Vibrio cholerae contains multiple copies of chemotaxis response regulator (VcCheY1–VcCheY4) whose functions are elusive yet. Autophosphorylated CheA then donates phosphate to the response regulator CheY. Phosphorylated CheY interacts with the flagellar motor protein FliM and influence the direction of flagellar rotation from counter clock wise (CCW) to clock wise (CW). As expected, both VcCheY3 and VcCheY4 possess (β/α)5 fold typical of the response regulators.

VcCheY4 was crystallized in two different states; one is in free state with no ligand attached (VcCheY4free) and another with a sulfate and a Ca2+ ion bound at the active site (VcCheY4sulf). In contrast to that, neither a metal ion nor a sulfate ion was observed at the active site of VcCheY4free although both of these components were added during crystallization. Absence of the divalent metal ion do not cause any change in the side chain conformation of D9 and D52 compared to VcCheY4sulf, but the carbonyl oxygen of N54 points away from the metal binding side. As a result, the β3α3 loop of VcCheY4free takes a different conformation and moves about 3 Å away from the active site. In VcCheY4free, helix α4 is shorter and β4α4 loop is unusually longer compared to those of VcCheY4sulf. The plot of B′-values indicated that the crystallographic B-factor of the β4α4 loop is much lower in VcCheY4sulf compared to that of VcCheY4free. Interestingly, when VcCheY4free is superposed on VcCheY4sulf significant differences are observed at the active site, together with helix α4, β4α4 loop and β3α3 loop. Our packing analysis suggests that, in either case, these regions are rather loosely packed and their conformations are not influenced by crystal packing. The crucial residue at β5 that acquires ‘in’ position upon activation is a Trp (W101) in case of VcCheY4 and in both the structures of VcCheY4 the side chain of W101 acquired ‘in’ position. In fact, this is the first structure of a naturally occurring CheY where Trp at this crucial position is observed to spontaneously occupy ‘in’ position, even without activation.

> TMAKVLAVDDSISIRQMVSHTLQDAGYEVETAADGREALAKAQKARFDVIISDVNMPVMTGFEFVKAVRMQSQYKFTPILMLTTETSPEKKQEGKAVGATGWLVKPFNPETLLKTLQRVL> MPFVNKQFNYKDPVNGVDIAYIKIPNAGQMQPVKAFKIHNKIWVIPERDTFTNPEEGDLNPPPEAKQVPVSYYDSTYLSTDNEKDNYLKGVTKLFERIYSTDLGRMLLTSIVRGIPFWGGSTIDTELKVIDTNCINVIQPDGSYRSEELNLVIIGPSADIIQFECKSFGHEVLNLTRNGYGSTQYIRFSPDFTFGFEESLEVDTNPLLGAGKFATDPAVTLAHELIHAGHRLYGIAINPNRVFKVNTNAYYEMSGLEVSFEELRTFG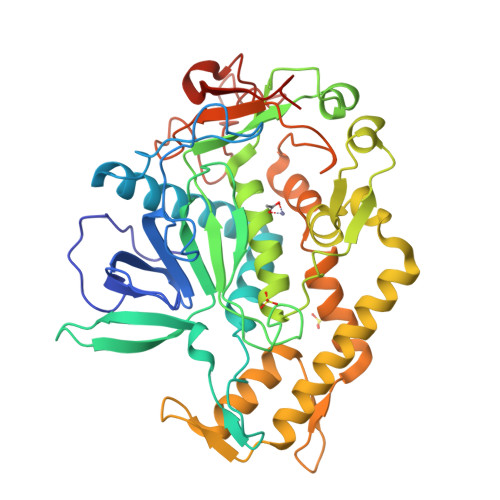GHDAKFIDSLQENEFRLYYYNKFKDIASTLNKAKSIVGTTASLQYMKNVFKEKYLLSEDTSGKFSVDKLKFDKLYKMLTEIYTEDNFVKFFKVLNRKTYLNFDKAVFKINIVPKVNYTIYDGFNLRNTNLAANFNGQNTEINNMNFTKLKNFTGLFELEHHHHHH Magnesium chelatase is a conserved enzyme complex responsible for the first committed step of chlorophyll biosynthesis in photosynthetic organisms, which is the addition of magnesium to the chlorophyll precursor, protoporphyrin IX. The complex is composed of the catalytic subunit ChlH, the bridging subunit ChlD, and the subunit ChlI, which serves as the motor that drives the entire complex. The motor subunit ChlI belongs to the superfamily of AAA+ (ATPases associated with diverse cellular activities) proteins and, through binding and hydrolyzing of ATP, provides the energy for the thermodynamically unfavorable reaction of Mg2+ insertion into protoporphyrin IX. Here, we used a combination of cryo-EM and functional analysis to investigate the mechanism of the ChlI motor subunit of magnesium chelatase from the cyanobacterium Nostoc sp. PCC 7120 (hereafter, Nostoc).

Iterative rounds of 3D classification, performed by multiple-class ab initio reconstructions followed by heterogeneous refinements, revealed two distinct classes, which we named hexamer conformations A and B. These reconstructions achieved global resolutions of 4 Å and 3.8 Å, respectively, with much greater local resolutions in the central parts of the structures. Conformation A is characterized by ATP molecules bound in five monomers and ADP in one, while conformation B has ATP bound in four monomers and ADP in two. Interestingly, each monomer contains a bound nucleotide molecule (ATP or ADP) in both hexameric states. Our reconstructions with no symmetry imposed revealed structural differences between the constituent monomers within the ring. Notably, the region of the insertions displayed varying levels of structural organization among the monomers. In the hexamer structures, the nucleotide state of each monomer is related to the structural organization of the insertions of that monomer, such that when an ATP molecule is bound, the insertions are folded and in an upward position. If ADP is bound, the inserts of this monomer are more flexible or even unfold, as demonstrated by fuzzy or absent corresponding cryo-EM densities. In contrast, in most ATP-bound states in our maps, these side chains are oriented toward the nucleotide (insets 1–3). Nevertheless, we cannot completely exclude the possibility that the nucleotide densities also correspond to mixtures of nucleotide states, for example, the density at monomer five in hexamer conformation A. Furthermore, in our ChlI hexamers, the monomers are pulled together in the upper region where the insertions are located, making the Nostoc ChlI ring more compact in contrast to Synechocystis.

>[6x]MHHHHHHTPTAQTTASARRVVFPFTAIVGQEEMKLALLLNVIDPKIGGVMIMGDRGTGKSTTIRALADLLPEIPVVANDPFNSDPSDPDLMSDEVRQKSGTGAEIPIEFKKVQMVDLPLGATEDRVCGTIDIEKALSEGVKAFEPGLLAKANRGILYVDEVNLLDDHLVDVLLDSAASGWNTVEREGISIRHPARFVLVGSGNPEEGELRPQLLDRFGMHAEIHTVKEPALRVQIVEQRSEFDQNPPTFLEKYNPEQTALQKKIVEAQKLLPEVKLDYDLRVKISEVCSELDVDGLRGDIVTNRAAKALTAYEGRTEVTVDDIRRVITLCLRHRLRKDPLESIDSGYKVEKVFARIFGVELLEDDSSQKNGAGQIKTGVR> MADLMMRRGEIWQVDLDPARGSEANNQRPAV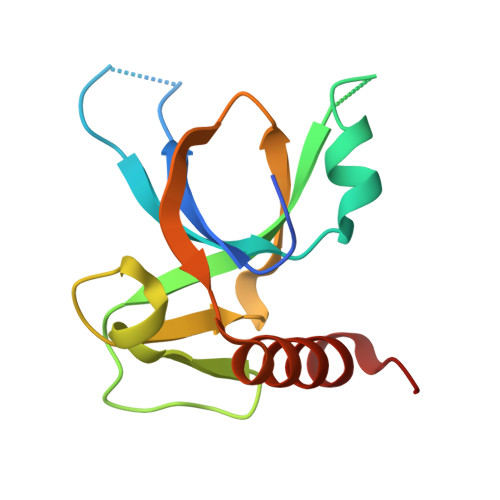VVSNDRANATATRLGRGVITVVPVTSNIAKVYPFQVLLSATTTGLQVDCKAQAEQIRSIATERLLRPIGRVSAAELAQLDEALKLHLDLWS> MQKRIALSFPEEVLEHVFSFIQLDKDRNSVSLVCKSWYEIERWCRRKVFIGNCYAVSPATVIRRFPKVRSVELKGKPHFADFNLVPDGWGGYVYPWIEAMSSSYTWLEEIRLKRMVVTDDCLELIAK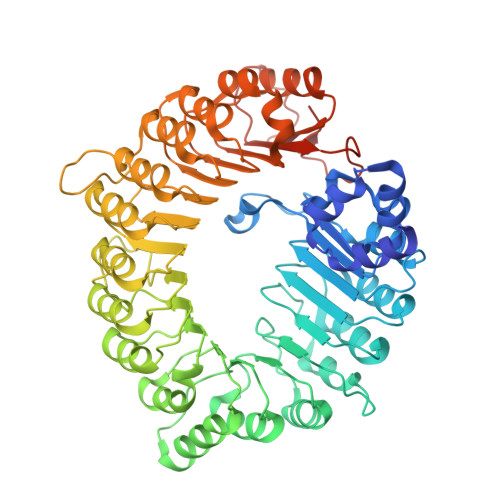SFKNFKVLVLSSCEGFSTDGLAAIAATCRNLKELDLRESDVDDVSGHWLSHFPDTYTSLVSLNISCLASEVSFSALERLVTRCPNLKSLKLNRAVPLEKLATLLQRAPQLEELGTGGYTAEVRPDVYSGLSVALSGCKELRCLSGFWDAVPAYLPAVYSVCSRLTTLNLSYATVQSYDLVKLLCQCPKLQRLWVLDYIEDAGLEVLASTCKDLRELRVFPSEPFVMEPNVALTEQGLVSVSMGCPKLESVLYFCRQMTNAALITIARNRPNMTRFRLCIIEPKAPDYLTLEPLDIGFGAIVEHCKDLRRLSLSGLLTDKVFEYIGTYAKKMEMLSVAFAGDSDLGMHHVLSGCDSLRKLEIRDCPFGDKALLANASKLETMRSLWMSSCSVSFGACKLLGQKMPKLNVEVIDERGAPDSRPESCPVERVFIYRTVAGPRFDMPGFVWNMDQDSTMRFSRQIITTNGL5-hydroxy-N-(1-oxo-1H-isoindol-6-yl)-1-(3-{[(phenylcarbamoyl)amino]methyl}phenyl)-1H-pyrazole-4-carboxamide 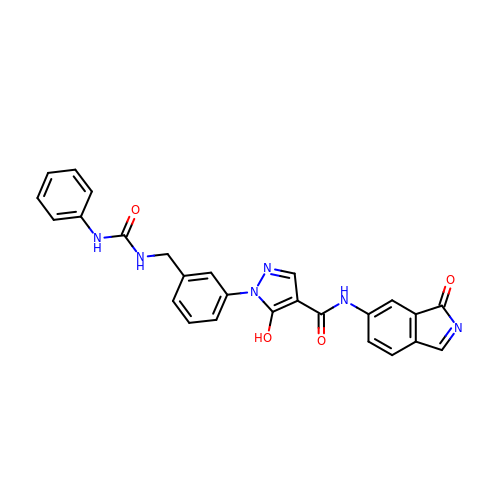| C26 H20 N6 O4 | UBLPJURRUDREKS-UHFFFAOYSA-N> 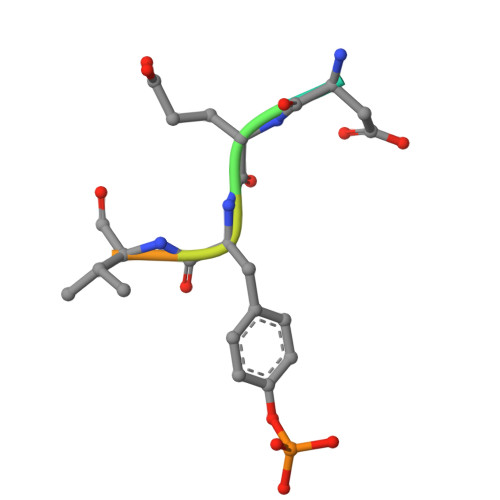LDEYVATR> MSNPLFPTESAALTLDGPVGPLDVAVDLPEPDVAVQPVTAIVCHPLSTEGGSMHNKVVTMAARALRELGITVVRFNFRSVGTSAGSFDHGDGEQ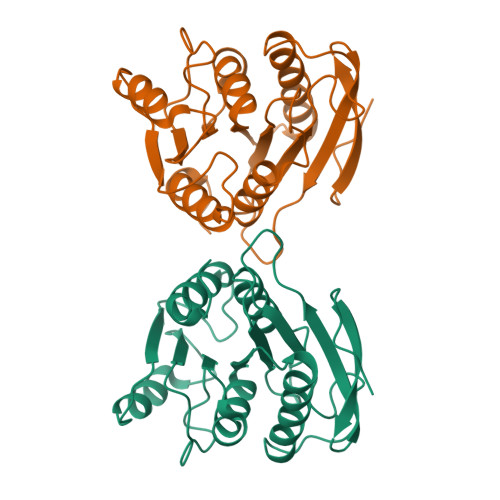DDLRAVAEWVRAQRPTDTLWLAGFSFGAYVSLRAAAALEPQVLISIAPPAGRWDFSDVQPPAQWLVIQGDADEIVDPQAVYDWLETLEQQPTLVRMPDTSHFFHRKLIDLRGALQHGVRRWLPATP> MNLRKRNELKSLFKNKSRLSETYFVELIDSTLNKRDDRFHGIWKP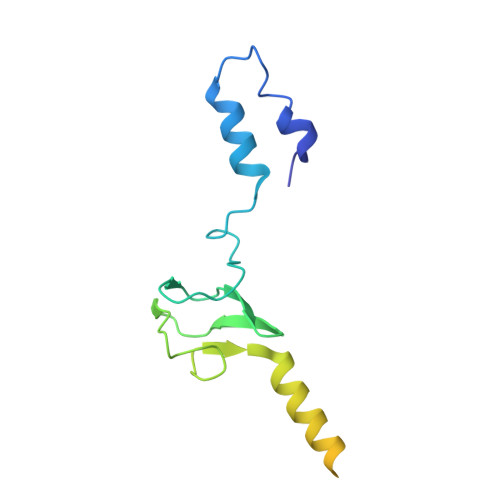GQTYQKGDVVYYNHSLWEMQSENEICAKEEQTPGISTDWKSLLKELEQKVDKLQHELETLHQEFTEYQKQMEIRLQLLARFIPILFIGLGIMFFWLLGQSTVHILAGTT> GA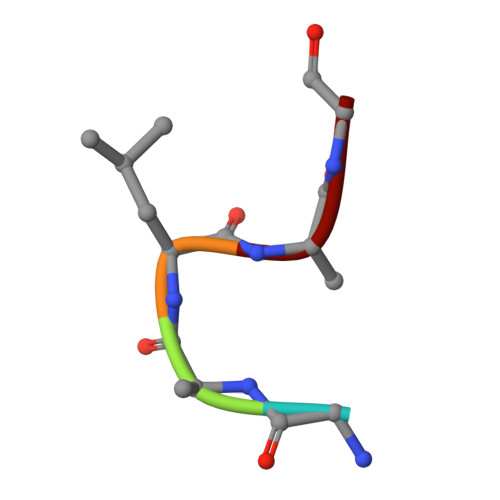LAG>[2x]NLNPAGSGSNSSAAGIAASMVGSPYVWGGSSPAGFDCSGLTSYAYAQAGISIPRTA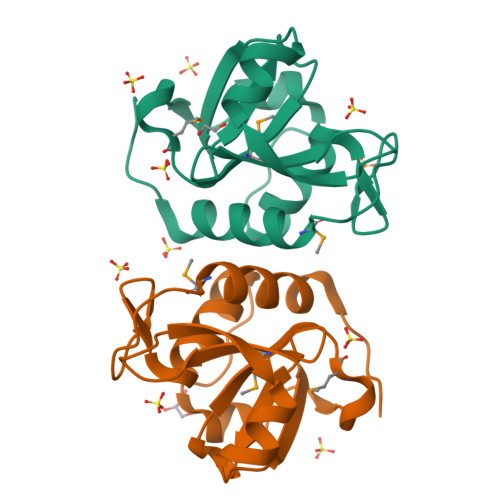GGQASVGSAVSYGNMQPGDLIVWSGGAHVSIYVGGGQMVHATNPSTGVITSSVSFWSNNSGQSITAIRRP4,4'-(ethylenediimino)bis[4-oxobutyrate] | C11 H18 N2 O6 | 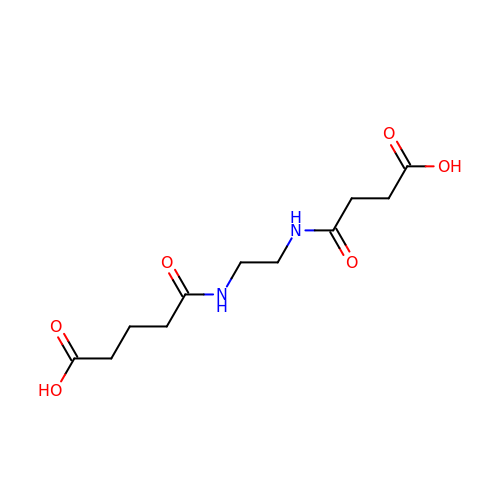JUHMDCQKNGDTCV-UHFFFAOYSA-N>PNMLNLLSNVETSLYEIQMLNYKY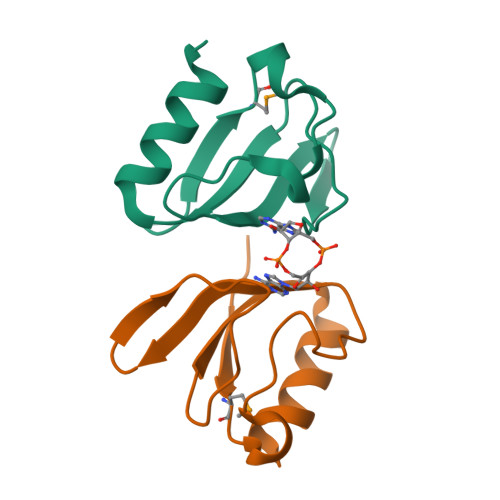ENIQLRNFPFGGDIIFVRIIRNNESIVPHGDTQLRYGDRLIVTGAKEYVDELKQELEFYF[2x]[(2~{S},3~{R},4~{R})-5-[8-methanoyl-7-methyl-2,4-bis(oxidanylidene)-1~{H}-benzo[g]pteridin-10-ium-10-yl]-2,3,4-tris(oxidanyl)pentyl] dihydrogen phosphate | C17 H20 N4 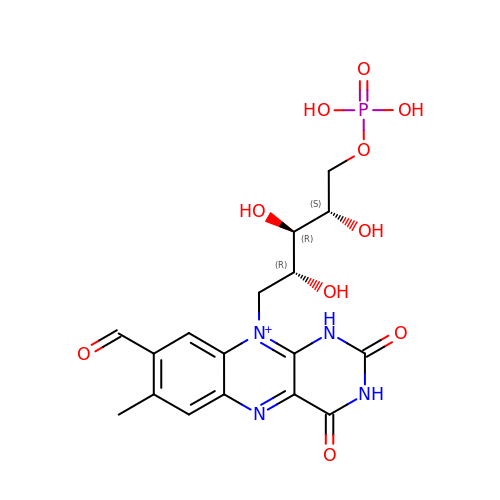O10 P | TZAPMZFMEMVUSE-MBNYWOFBSA-O>[2x]MAYPGHPGAGG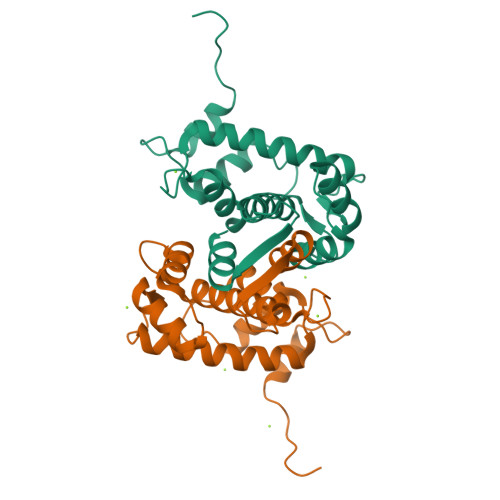GYYPGGYGGAPGGPAFPGQTQDPLYGYFAAVAGQDGQIDADELQRCLTQSGIAGGYKPFNLETCRLMVSMLDRDMSGTMGFNEFKELWAVLNGWRQHFISFDTDRSGTVDPQELQKALTTMGFRLSPQAVNSIAKRYSTNGKITFDDYIACCVKLRALTDSFRRRDTAQQGVVNFPYDDFIQCVMSV The earliest discovered selective autophagy pathway in Saccharomyces (S.) cerevisiae is the cytoplasm‐to‐vacuole targeting (Cvt) pathway, through which hydrolytic enzymes are sequestered into double‐membrane vesicles, termed Cvt vesicles, and transported to the vacuole 8, 9. The best‐characterized cargo component of the Cvt vesicle is the vacuolar aminopeptidase I (Ape1) 16. Ape1 is synthesized in the cytosol as a 55‐kDa zymogen that includes an N‐terminal propeptide (hereafter referred to as prApe1), which oligomerizes into a dodecamer 17, 18 and further assembles into larger aggregates in a propeptide‐dependent manner 19. In addition to prApe1, Atg19 also binds another cargo hydrolase α‐mannosidase 1 (Ams1) 25, 26 via a site distinct from the prApe1 binding site, thus forming the Cvt complex.

When expressing S. cerevisiae mApe1 (sc‐mApe1) lacking the N‐terminal propeptide, we predominantly observed isolated dodecamers when imaged at identical protein concentration and buffer conditions, indicating that the propeptide stimulates the trans‐interactions between multiple prApe1 dodecamers. Due to the presence of smaller particles of putative mApe1 hexamers (white arrowheads), we stabilized and purified sc‐mApe1 using a GraFix gradient 29. Based on the twofold and threefold end‐on views from class average analysis, we determined a low‐resolution negative stain structure at 24 Å resolution by imposing tetrahedral symmetry (and EV1E). Class averages of sc‐mApe1 dodecamers including views of twofold and threefold symmetry. Fourier shell correlation of the EM reconstruction of the sc‐mApe1 dodecamer indicates a resolution of 24 Å. In the crystal, ct‐mApe1 is present as dodecamers, which are formed by two asymmetric units each containing six ct‐mApe1 molecules. The ct‐mApe1 X‐ray structure is compatible with the dimensions of the sc‐mApe1 EM projections and fits very well into the tetrahedral low‐resolution EM density (Figs 1G and EV2). Comparison of twofold and threefold views (left and right) of the determined 24 Å resolution EM map of Saccharomyces cerevisiae mApe1 (sc‐mApe1) (upper row) with the simulated 24 Å resolution map of the ct‐mApe1 X‐ray crystal structure (lower row) shows very close visual agreement. A black sphere represents the N‐terminus where the propeptide would emanate from the dodecamer. Moreover, the geometric positioning of the N‐terminal propeptide on the surface of the dodecamer is consistent with our observed trans‐interactions of dodecamers leading to higher‐order assemblies.

> MEEQREILEQLKKTLQMLTVEPSKNNQIANEEKEKKENENSWCILEHNYEDIAQEFIDFIYKNPTTYHVVSFFAELLDKHNFKYLSEKSNWQDSIGEDGGKFYTIRNGTNLSAFILGKNWRAEKGVGVIGSHVDALTVKLKPVSFKDTAEGYGRIAVAPYGGTLNELWLDRDLGIGGRLLYKKKGTNEIKSALVDSTPLPVCRIPSLAPHFGKPAEGPFDKEDQTIPVIGFPTPDEEGNEPPTDDEKKSPLFGKHCIHLLRYVAKLAGVEVSELIQMDLDLFDVQKGTIGGIGKHFLFAPRLDDRLCSFAAMIALICYAKDVNTEESDLFSTVTLYDNEEIGSLTRQGAKGGLLESVVERSSSAFTKKPVDLHTVWANSIILSADVNHLYNPNFPEVYLKNHFPVPNVGITLSLDPNGHMATDVVGTALVEELARRNGDKVQYFQIKNNSRSGGTIGPSLASQTGARTIDLGIAQLSMHSIRAATGSKDVGLGVKFFNGFFKHWRSVYDEFGEL> SAKDPMDRAAHAVEQWRSERPDLDPSSMIVLGRLQEAALVIARDRLNPLFARYGLQPGEFDVLATLRRSGAPYALTPTALYDAAMISSGSMTNRIDRLEKAGWVERRANPADGRGTLVALTSAGRALIDDAVVAHVDNQRRVLSALSAAEQRQLA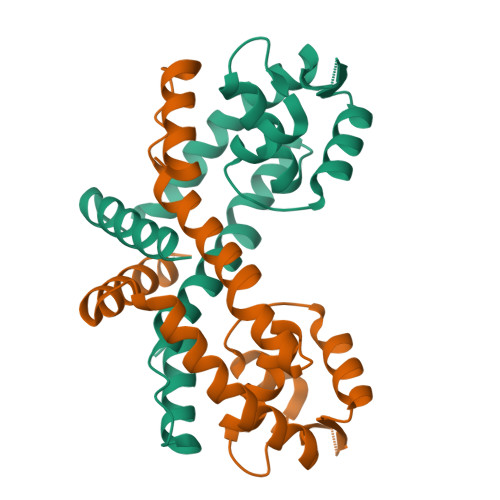KLLDKLLQGQAAEG>MGRIKNKQFAVIGLGAFGGSICKELHRMGHEVLAVDINEEKVNAYASYATHAVIANATEENELLSLGIRNFEYVIVAIGANIQASTLTTLLLKELDIPNIWVKAQNYYHHKVLEKIGADRIIHPEKDMGVKIAQSLSDENVLNYIDLSDEYSIVELLATRKLDS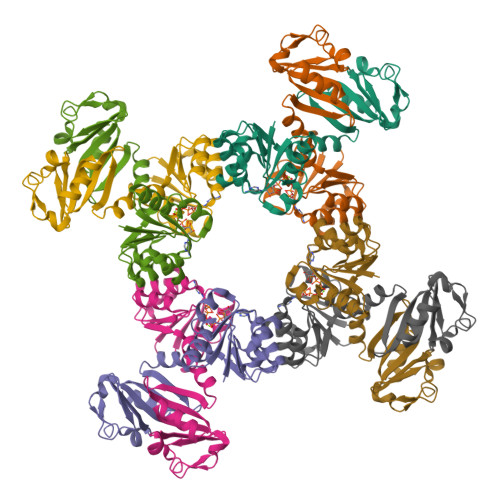KSIIDLNVRAKYGCTILAIKHHGDICLSPAPEDIIREQDCLVIMGHKKDIKRFENEGM[2x]>MMPIKSIVTLDQLEDSEYLFRIVSTVLPHLCLDYKVCDQLKTTFVHPFDILLNNSLGSVTKQDELQAAISKLGINYLIDTTSRELKLFNVTLNAGNIDIINTPINISSETNPIINTHSFYDLPPFTQHLLNIRLTDTEYRARFIGGYIKPDGSDSMDVLAEKKYPDLNFDNTYLFNILYKDVINAPIKEFKAKIVNGVLSRQDFDNLIGVRQYITIQDRPRFDDAYNIADAARHYGVNLNTLPLPNVDLTTMPTYKHLIMFEQYFIYTYDRVDIYYNGNKMLFDDEIINFTISMRYQSLIPRLVDFFPDIPVNNNIVLHTRDPQNAAVNVTVALPNVQFVDINRNNKFFINFFNLLAKEQRSTAIKVTKSMFWDGMDYEEYKSKNLQDMMFINSTCYVFGLYNHNNTTYCSILSDIISAEKTPIRVCLLPRVVGGKTVTNLISETLKSISSMTIREFPRKDKSIMHIGLSETGFMRFFQLLRLMADKPHETAIKEVVMAYVGIKLGDKGSPYYIRKESYQDFIYLLFASMGFKVTTRRSIMGSNNISIISIRPRVTKQYIVATLMKTSCSKNEAEKLITSAFDLLNFMVSVSDFRDYQSYRQYRNYCPRYFYAG[3x];>[3x]MDFFNKFSQGLAESSTPKSSIYYSEEKDPDTKKDEAIEIGLKSQESYYQRQLREQLARDNMTVASRQPIQPLQPTIHITPQPVPTATPAPILLPSSTVPTPKPRQQTNTSSDMSNLFDWLSEDTDAPASSLLPALTPSNAVQDIISKFNKDQKTTTPPSTQPSQTLPTTTCTQQSDGNISCTTPTVTPPQPPIVATVCTPTPTGGTVCTTAQQNPNPGAASQQNLDDMALKDLMSNVERDMHQLQAETNDLVTNVYDAREYTRRAIDQILQLVKGFERFQK

Vaccinia virus assembly in the cytoplasm of infected cells involves the formation of a biconcave viral core inside the maturing viral particle. The boundary of the core is defined by a pseudohexagonal palisade layer, composed of trimers projecting from an inner wall. In contrast, A4 and A10, which are essential for virion assembly, are accessible on the surface of intact viral cores suggesting that they are palisade components. Moreover, A10 and A4 form a stable complex that can be cross-linked in purified IMVs.

We obtained a palisade map at a subnanometer resolution, which reveals a trimeric structure as a single conformer. The trimer is ~13 nm in height and 8 nm in diameter and consists of a closely packed cylindrical base that sits on top of the inner core wall, with separated lobes projecting toward the viral membrane. We found that most of the density in our palisade map is unambiguously explained by a model of the processed N-terminal fragment 1 of A10. Ordered densities that would account for the C-terminal fragments 2 and 3 were not identified, suggesting that only fragment 1 of A10 is a structural component of the palisade trimer. While the trimer of processed A10 accounts for most of our STA map, an elongated density (~60 Å in length) on the exterior surface of each A10 molecule remained unexplained. An AlphaFold2 model of an A10/A4 heterodimer revealed that an alpha helix of A4 (residues 24–66) located in a groove in the A10 model predictably accounts for the unexplained density (Fig. 2B through D). Our maps, therefore, indicate that the palisade consists of an A10 trimer in which each protomer binds a long alpha helix located near the N-terminus of A4, where the N-terminus of this helix points toward the inner wall and the C-terminus points toward the viral membrane. Within the trimer, each A10 monomer consists of three regions: the A4-interacting domain (residues 169–364), which forms the projecting lobes at the apex of the trimer and mediates the interaction with A4; the medial domain (residues 38–168 and 365–431), which encloses a cavity in the center of the trimer base; and the inner wall-proximal domain (residues 1–37 and 432–614), which forms the base of the trimer and interacts with the inner core wall. In total, each inter-protomer interface consists of approximately 2,285 Å2 of the buried surface area. In addition, the A4 helix binding in the groove on A10 buries 1,220 Å2 of the surface area.>MKVKGLSVLVVCTGNLCRSPMAEIILRDKIRQKRLNIQVRSAGTLKTGKTMPDDKALQALQDYGYHPMVNPVQQVTQQDFIEHDFIYAMDRTNLADLLDICPAEHKNKLALFLSKANRQEKEVPDPYRRSSEFFQRTALLIESGAVAL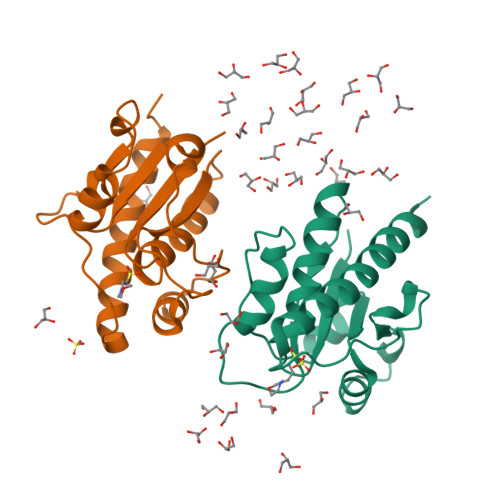VDSWQEQGINACNENLSQ[2x]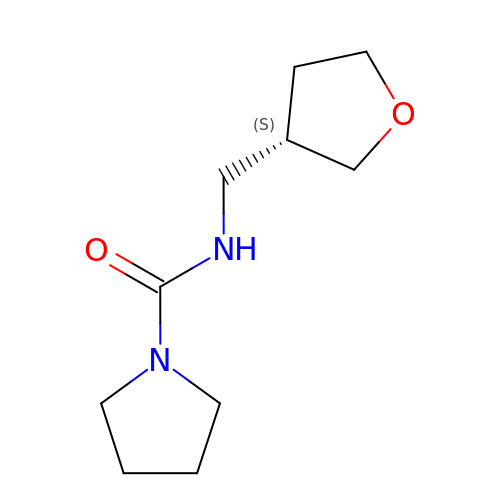N-{[(3S)-oxolan-3-yl]methyl}pyrrolidine-1-carboxamide | C10 H18 N2 O2 | MDOWUCLFMQLBNB-VIFPVBQESA-N> GAEGHIAHYDLNKLHSTSEAAVNKEHILILTPMQTFHQQYWDNLLQLNYPRELIELGFITPRTATGDLALKKLENAIKKVQTDKKTQRFSKITILRQNSQSFDKLMEKERHALDVQKERRAAMALARNELLFSTIGPHTSWVLWLNADIIETPPSLIQDMTKHNKAILAANIYQRFYDEEKKQPSIRPYDFNNWQESDTGLEIASQMGDDEIIVEGYAEIATYRPLMAHFYDANGVPGEEMALD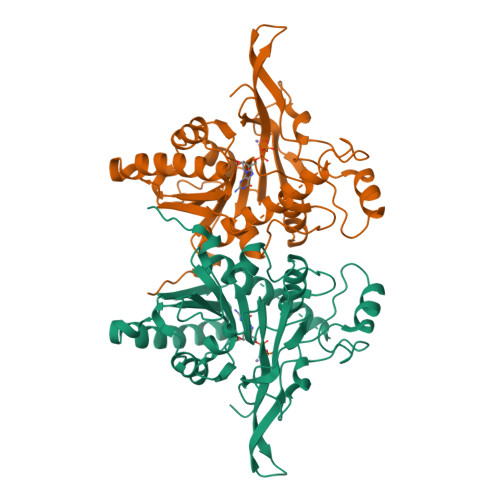GVGGGCTLVKAEVHRDGAMFPNFPFYHLIETEGFAKMAKRLNYDVFGLPNYLVYHIEEENH>GPLGSPEFELGTTEILRHSMDPPTFTFNFNNEPWVRGRHETYLCYEVERMHNDTWVKLNQRRGFLANQAPHKHGFLEGRHAELCFLDVIPFWKLDLDQDYRVTCFTSWSPCFSCAQEMAKFISKNKHVSLCIKTARIYDDQGRAQEGLRTLAEAGAKISIMTYSEFKHCWDTFVDHQGAPFQPWDGLDEHSQDLSGRLRAILQNQ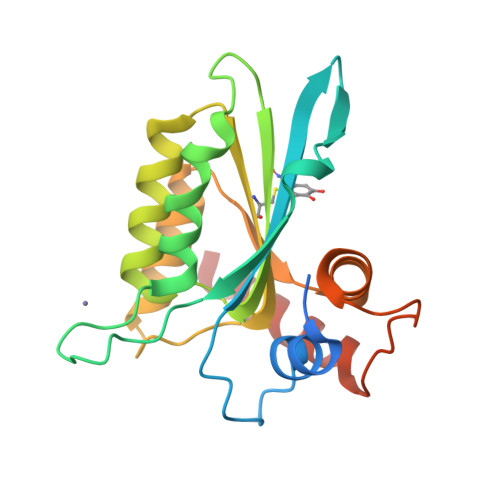EN[2x]PHOSPHORIC ACID MONO(FORMAMIDE)ESTER | C H4 N O5 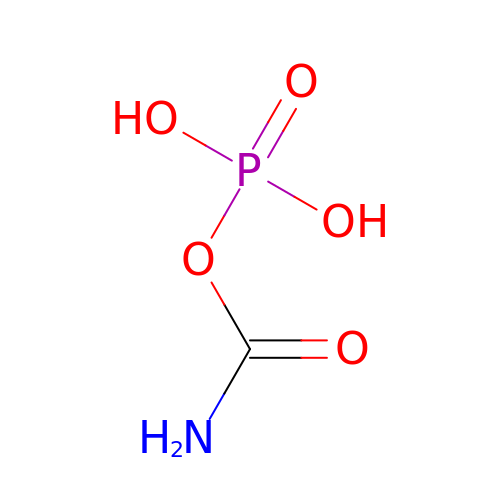P | FFQKYPRQEYGKAF-UHFFFAOYSA-N>MAVATDQVKTFLQKISHTNYIVRDHRVHQIRVLPGVTLIDMLYRLAAGYLGERPIELRQIIFKQPVVTSEEFDKHLYVTFTPARDSWKVEITSEKAKNGTPLGGNRDENMECQLYLQEDAPRAKELNIEAFMKNASRKWDMHDIYGIARRSHIEHGEFMKNEGAVYQLQDKEELMELTLSDLAEGFREKFKAHPAFLDASTLAGSSFALSAQKQNDTPYIPFMIDRFCMYQPFPKTIYTYSAKNSRTESGVSDSEPDVYSADFTIYDRAGNVLAECEKLTVKRVRQANM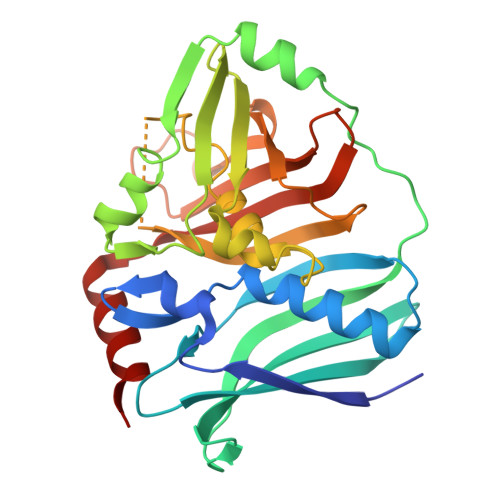ITHLEHHHHHH[4x]>[4x]MAHHHHHHSSGLEVLFQGPGHKKKLEGKVAIVTGGASGIGETAARIFADHGARAVVIADIQSELGRMVAESIGAKRCSYVQCDIADEEQVKSAVEWTATTYGGLDVMFCNAGIMSHSDSGQTVMELDMSKFDEVMRVNTRGTAACVKQAARKMVELGTRGGAIICTSSPLATRGGHVDTDYVMSKHAVLGLVRSASMQLGAHGIRVNSVSPMAVLTPLTRRMGLATPADVENALGRFTSLKGVALTAEHVAEAAAFLASDEAAFITGHDLVVDGGLLCLPFAAHS

1 is then reduced by the enzyme iridoid synthase (ISY), which generates a reactive intermediate 8-oxocitronellyl enol 2 that is primed to cyclize to form the canonical nepetalactol 3 scaffold, the precursor to all iridoids in plants. The stereochemistry of the bridgehead carbons (C4a and C7a) are set during the subsequent cyclization of 8-oxocitronellyl enol 2, the ISY product, to form 3. Some NEPS, although containing an NAD+ binding site, are redox inactive and catalyze only cyclization, others catalyze only the oxidation from nepetalactol to nepetalactone, while others are dual-function enzymes, catalyzing both stereo-selective cyclization and oxidation of various nepetalactols to nepetalactones. Here, we set out to understand and expand the selectivity of NEPS by both gene discovery in Nepeta sibirica and enzyme engineering of NEPS from various Nepeta species: N. sibirica, N. cataria and N. mussinii.

We identified, characterized and subjected to crystallography analysis the NEPS orthologue NsNEPS2 as a 7S-cis-trans nepetalactone 4a synthase. Biochemical assays showed that NsNEPS2 (N. sibirica) is a cis-trans cyclase and oxidase; when NsNEPS2 is incubated with 8-oxogeranial 1 and 7S-ISY, 7S-cis-trans nepetalactone 4a, with no presence of iridodial 5 byproducts, is observed. Since NEPS belong to the NAD+-dependent short chain dehydrogenase family, mutation of the active site tyrosine residue required for oxidation in this class of enzymes could be a straightforward way to decouple cyclization and oxidative activity. Mutation of the active site tyrosine in NsNEPS2 (NsNEPS2-Y167F) yielded an enzyme that produces only 7S-cis-trans nepetalactol 3a, with no iridodial 5 byproducts, suggesting that cyclization activity was maintained while oxidation activity was eliminated. NsNEPS2, 7S-cis-trans nepetalactone 4a synthase when assayed with 7S-ISY, yielded 7R-cis-trans nepetalactone 4a’ when assayed with 7R-ISY. Correspondingly, NsNEPS2-Y167F yielded 7R-cis-trans nepetalactol 3a’. In summary, the active site of NsNEPS2 can accommodate formation of both enantiomers, 7R-cis-trans 4a and 7S-cis-trans 4a’ which have two unique 4a-7a bridge configurations (4aR,7aS vs. 4aS,7aR, respectively). NsNEPS2 is able to catalyze cyclization of enantiomers yielding cis-trans stereochemistry for both 7 S and 7 R ISY. Enzyme assays with 8-oxogeranial and NsISY show that NsNEPS1A, NsNEPS1B, NsNEPS2 and NsNEPSL all oxidize 7S-cis-trans nepetalactol 3a to 7S-cis-trans nepetalactone 4a. Based on the available NEPS crystal structures (NmNEPS3 and NsNEPS2), we hypothesized that the relatively bulky L199 residue in NmNEPS4 prevents the orientation of the 3c relative to the NAD+ cofactor required for oxidation.> RQLALEAKGETPSAV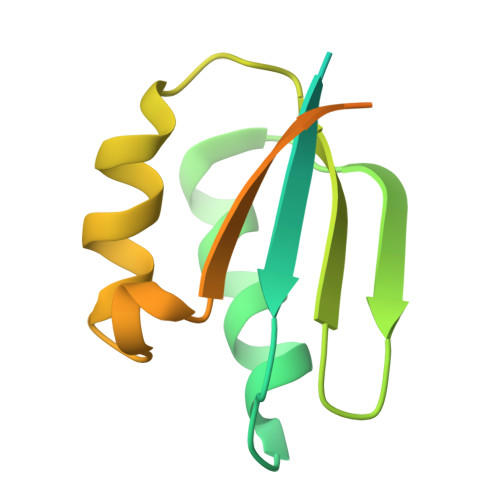TRLSVVAKSEPQDEQSRSQSPRRIILSRLKAGEVDLLEEELGHLTTLTDVVKGADSLSAILPGDIAEDDITAVLCFVIEADQITFETVEVSPKISTPPVLKLAAEQAPTGRVEREKTTR NAD+ synthetase can be either monofunctional ammonia-dependent NAD+ synthetase using uniquely free ammonia as a substrate or multifunctional glutamine-dependent NAD+ synthetase (glnNAD+ synthetase) using glutamine as the source of ammonia. glnNAD+ synthetase catalyzes the ATP-dependent formation of NAD+ from nicotinic acid adenine dinucleotide (NaAD+) at the synthetase domain using the ammonia generated from the glutaminase domain21. Here, we report the structural and kinetic characterizations of hsNadE and a direct structural comparison of the closed and active conformation of (1) hsNadE structure in complex with a synthetase intermediate analog at 2.84 Å resolution and (2) tbNadE structure in complex with glutamine, sulfonamide derivative 1 (5′-O-(N-(nicotinyl)sulfamoyl) adenosine; SFI), and PPi at 3.14 Å resolution. Both structures are snapshots of the enzymes in the allosteric state with the synthetase active site loop ordered revealing an exclusive rearrangement of the glutaminase active site and the molecular tunnels.

As predicted from the kinetic data showing 16-fold activation of the glutaminase domain when the synthetase domain is occupied by SFI and MgPPi, co-crystallization of tbNadE with SFI, MgPPi, and glutamine trapped the enzyme in the closed activated conformation. In this crystal structure, we found one SFI molecule occupying the NaAD+-binding site and another SFI along with PPi bound in ATP-binding site (SFI-1 and SFI-2, respectively). Closure of the P2 loop observed in subunit Bsyn reveals two close contacts, the first between the P2 loop residue Glu552TB and N-(nicotinyl)sulfamoyl linkage of SFI bound in the ATP-binding site (SFI-2), and the second between the one O atoms of PPi and Glu541TB, a terminal residue of α16 adjacent to P2 loop. The nicotinic ring like moiety of the SFI bound in the NaAD+-binding site is highly flexible due to the absence of protein–ligand interactions. PPi was built only in the synthetase active site of subunit B with the P loops ordered (partial occupancy of 0.58). No Mg2+ could be identified in this complex due to a partial occupancy of PPi. The binding of SFI in the ATP-binding site and MgPPi at the synthetase active site leads to the ordering of the P2 loop (in subunit Bsyn) and rearrangement of the glutaminase active site to trap in a non-productive mode (Gln-NP) the glutamine substrate in its coupled active site (in subunit Dglu). Interestingly, the ordering of the P loops in subunit Bsyn (and symBsyn in octamer) could induce a productive binding mode of glutamine (Gln-P) activating the glutaminase active site in the uncoupled active site (Cglu and symCglu Fig. 3g).

>MNFYSAYQHGFVRVAACTHHTTIGDPAANAASVLDMARACHDDGAALAVFPELTLSGYSIEDVLLQDSLLDAVEDALLDLVTESADLLPVLVVGAPLRHRHRIYNTAVVIHRGAVLGVVPKSYLPTYREFYERRQMAPGDGERGTIRIGGADVAFGTDLLFAASDLPGFVLHVEIAEDMFVPMPPSAEAALAGATVLANLSGSPITIGRAEDRRLLARSASARCLAAYVYAAAGEGESTTDLAWDGQTMIWENGALLAESERFPKGVRRSVADVDTELLRSERLRMGTFDDNRRHHRELTESFRRIDFALDPPAGDIGLLREVERFPFVPADPQRLQQDCYEAYNIQVSGLEQRLRALDYPKVVIGVSGGLDSTHALIVATHAMDREGRPRSDILAFALPGFATGEHTKNNAIKLARALGVTFSEIDIGDTARLMLHTIGHPYSVGEKVYDVTFENVQAGLRTDYLFRIANQRGGIVLGTGDLSELALGWSTYGVGDQMSHYNVNAGVPKTLIQHLIRWVISAGEFGEKVGEVLQSVLDTEITPELIPTGEEELQSSEAKVGPFALQDFSLFQVLRYGFRPSKIAFLAWHAWNDAERGNWPPGFPKSERPSYSLAEIRHWLQIFVQRFYSFSQFKRSALPNGPKVSHGGALSPRGDWRAPSDMSARIWLDQIDREVPKG[4x]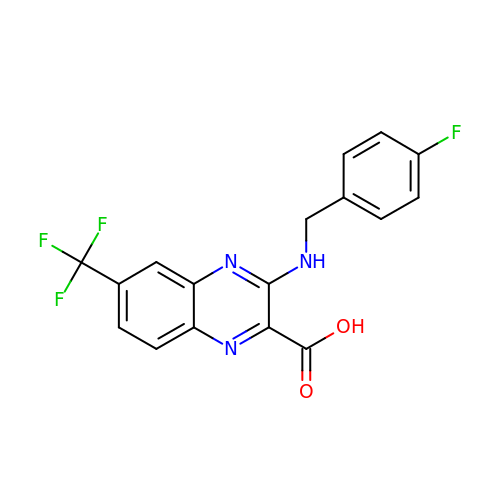3-[(4-fluorobenzyl)amino]-6-(trifluoromethyl)quinoxaline-2-carboxylic acid | C17 H11 F4 N3 O2 | HUDWVBGXXJRCNV-UHFFFAOYSA-N>[4x]TELTLKPGTLTLAQLRAIHAAPVRLQLDASAAPAID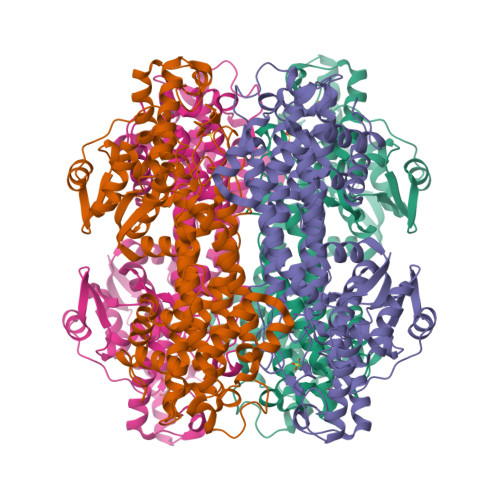ASVACVEQIIAEDRTAYGINTGFGLLASTRIASHDLENLQRSLVLSHAAGIGAPLDDDLVRLIMVLKINSLSRGFSGIRRKVIDALIALVNAEVYPHIPLKGSVGASGDLAPLAHMSLVLLGEGKARYKGQWLSATEALAVAGLEPLTLAAKEGLALLNGTQASTAYALRGLFYAEDLYAAAIACGGLSVEAVLGSRSPFDARIHEARGQRGQIDTAACFRDLLGDSSEVSLSHKNADKVQDPYSLRCQPQVMGACLTQLRQAAEVLGIEANAVSDNPLVFAAEGDVISGGNGHAEPVAMAADNLALAIAEIGSLSERRISLMMDKHMSQLPPFLVENGGVNSGFMIAQVTAAALASENKALSHPHSVDSLPTSANQEDHVSMAPAAGKRLWEMAENTRGVLAIEWLGACQGLDLRKGLKTSAKLEKARQALRSEVAHYDRDRFFAPDIEKAVELLAKGSLTGLLPAGVLPSL>MDMGISGKVAVITGSSSGIGLAIAEGFAKEGAHIVLVARQVDRLHEAARSLKEKFGVRVLEVAVDVATPEGVDAVVESVRSSFGGADILVNNAGTGSNETIMEAADEKWQFYWELHVMAAVRLARGLVPGMRARGGGAIIHNASICAVQPLWYEPIYNVTKAALMMFSKTLATE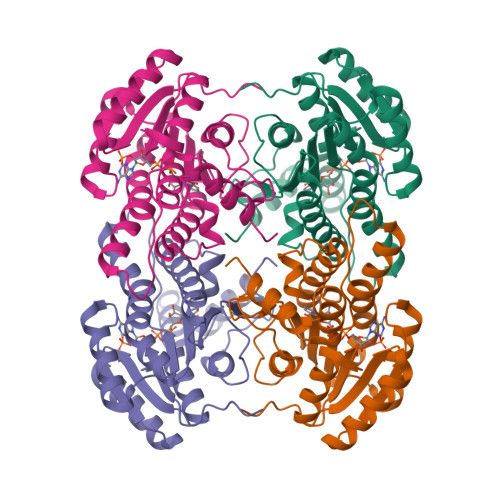VIKDNIRVNCINPGLILTPDWIKTAKELTKDNGGDWKGYLQSVADEHAPIKRFASPEELANFFVFLCSERATYSVGSAYFVDGGMLKTL[8x]>[2x]MEEVVIAGMSGKLPESENLQEFWDNLIGGVDMVTDDDRRWKAGLYGLPRRSGKLKDLSRFDASFFGVHPKQAHTMDPQLRLLLEVTYEAIVDGGINPDSLRGTHTGVWVGVSGSETSEALSRDPETLVGYSMVGCQRAMMANRLSFFFDFRGPSIALDTACSSSLMALQNAYQAIHSGQCPAAIVGGINVLLKPNTSVQFLRLGMLSPEGTCKAFDTAGNGYCRSEGVVAVLLTKKSLARRVYATILNAGTNTDGFKEQGVTFPSGDIQEQLIRSLYQSAGVAPESFEYIEAHGTGTKVGDPQELNGITRALCATRQEPLLIGSTKSNMGHPEPASGLAALAKVLLSLEHGLWAPNLHFHSPNPEIPALLDGRLQVVDQPLPVRGGNVGINSFGFGGSNVHIILRPNTQ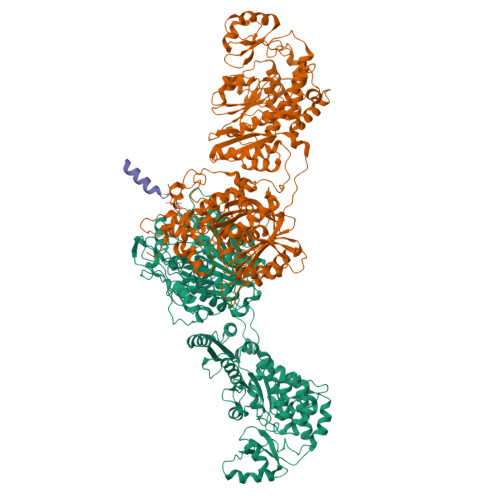PPPAPAPHATLPRLLRASGRTPEAVQKLLEQGLRHSQDLAFLSMLNDIAAVPATAMPFRGYAVLGGERGGPEVQQVPAGERPLWFICSGMGTQWRGMGLSLMRLDRFRDSILRSDEAVKPFGLKVSQLLLSTDESTFDDIVHSFVSLTAIQIGLIDLLSCMGLRPDGIVGHSLGEVACGYADGCLSQEEAVLAAYWRGQCIKEAHLPPGAMAAVGLSWEECKQRCPPGVVPACHNSKDTVTISGPQAPVFEFVEQLRKEGVFAKEVRTGGMAFHSYFMEAIAPPLLQELKKVIREPKPRSARWLSTSIPEAQWHSSLARTSSAEYNVNNLVSPVLFQEALWHVPEHAVVLEIAPHALLQAVLKRGLKPSCTIIPLMKKDHRDNLEFFLAGIGRLHLSGIDANPNALFPPVEFPAPRGTPLISPLIKWDHSLAWDVPAAEDFPNGS;> DXLMSVEVRQTLEREL>MPLGLLWLGLALLGALHAQAQDSTSDLIPAPPLSKVPLQQNFQDNQFQGKWYVVGLAGNAILREDKDPQKMYATIYELKEDKSYNVTSVLFRKKKCDYAIATFVPGSQ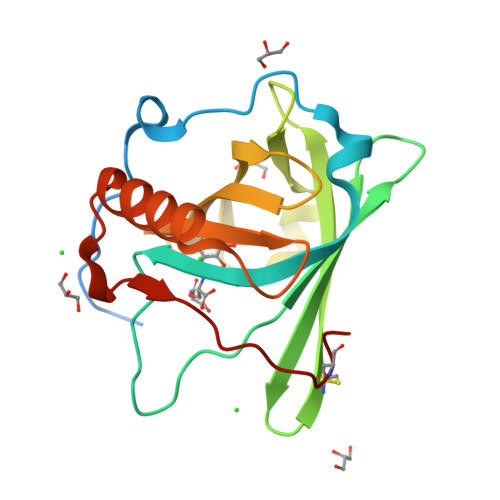PGEFTLGNIKSYPGLTSFLVRVVSTNYNQHAMVFFKKVSQNREYFKITLYGRTKELTSELKENFIRFSKSLGLPENHIVFPVPIDQCIDG[3x]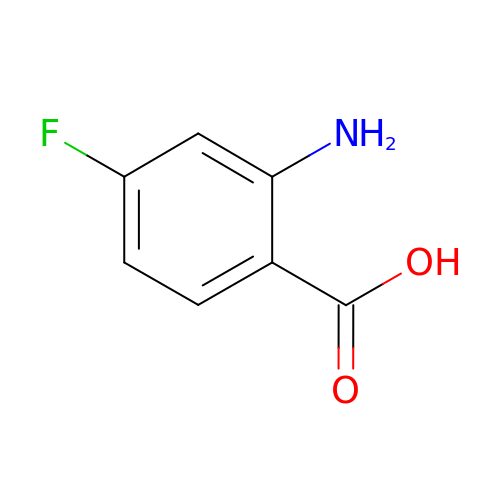2-amino-4-fluorobenzoic acid | C7 H6 F N O2 | LGPVTNAJFDUWLF-UHFFFAOYSA-N>[2x]MARKTIIAGNWKMNLSLKEAVFLAHSIREKIPSISKDKVSMVFPSTLHLENVSKILEGSSVIVGAQNCYHSGLAAFTGETSPDQLKEIGVKVVMVGHSERRQFLGESNFFCNDKIRFLLKNEFTVLYCVGETLSERESGKTLEVLSSQIREGLKGIDSVFFSNLILAYEPVWAIGTGKVATPSQAQEVHSFIRKEIS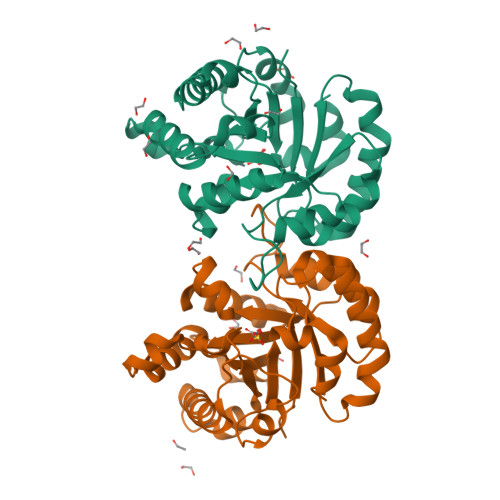GLFVGASSISESISILYGGSVKPDNIQDLLKEKDIDGGLVGGASQKISSFAGLF> MTVFRQENVDDYYDTGEELGSGQFAVVKKCREKSTGLQYAAKFIKKRRTKSSRRGVSREDIEREVSILKE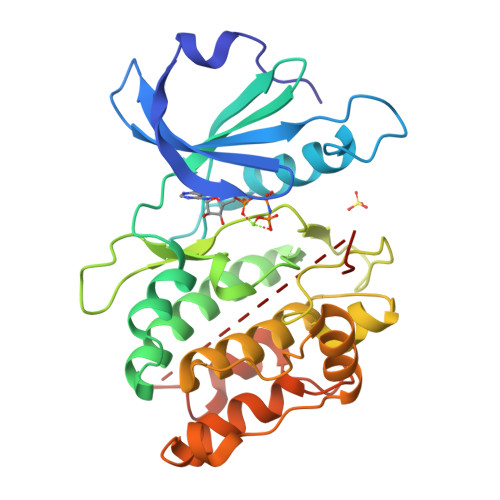IQHPNVITLHEVYENKTDVILILELVAGGELFDFLAEKESLTEEEATEFLKQILNGVYYLHSLQIAHFDLKPENIMLLDRNVPKPRIKIIDFGLAHKIDFGNEFKNIFGTPEFVAPEIVNYEPLGLEADMWSIGVITYILLSGASPFLGDTKQETLANVSAVNYEFEDEYFSNTSALAKDFIRRLLVKDPKKRMTIQDSLQHPWIKPKDTQQALSSAWSHPQFEK>GIDPFTVPLIFKIGYNVIPLQDVILPTPSSKVLKYLIQSGKLLPSLNNLITSRDKYKPIFISHLGLNQRRIFQTNGNLKTISRGSKLSSTIAFSTQVNVLPELDEGVFETIYGKFHITIESVEIVEVEKLKEEVEKHMNDNIRVRFISPTLLSSKVLLPPSLSERYKRVNAGYSTLPSVGLIVAY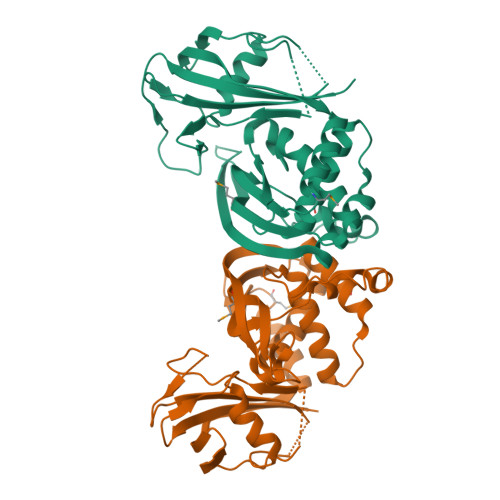AYNVYCNLIGKKEVEVRAFKFGVISNALSRIIGYDLHPVTIVIGEDSKGNLRKARGVMGWIEFDIPDEKLKRRALRYLLASSYLGIGRSRGIGFGEIKLEFIKREENH[4x]(2~{R})-6,6,9,9-tetramethylspiro[3,4,7,8-tetrahydrobenzo[g]chromene-2,2'-3,4-dihydrochromene]-6'-carboxylic 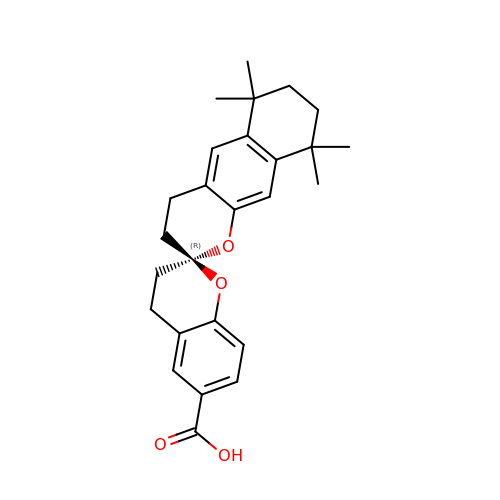acid | C26 H30 O4 | BWUCHLRCLVDMCC-SANMLTNESA-N N-(1-{3-[2-(2-amino-3-{3-[(3,3-dimethylbutyl)amino]-3-oxopropyl}quinolin-6-yl)phenyl]prop-2-yn-1-yl}cyclopropyl)-4-fluorobenzamide | C37 H39 F N4 O2 | 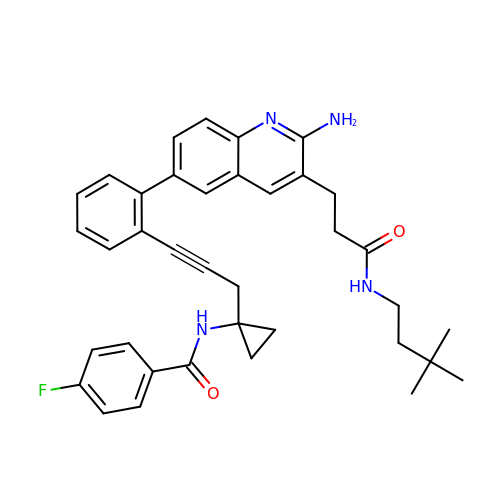QLQWEADMFLXRFH-UHFFFAOYSA-N>MAKKTGAKYPKSLLSLPLVGSLPFLPRHGHMHNNFFKLQKKYGPIYSVRMGTKTTVIVGHHQLAKEVLIKKGKDFSGRPQMATLDILSNNRKGIAFADSGAHWQLHRRLAMATFALFKDGDQKLEKIICQEISTLCDMLATHNGQSIDISFPVFVAVTNVISLICFNTSYKNGDPELNVIQNYNEGIIDNLSKDSLVDLVPWLKIFPNKTLEKLKSHVKIRNDLLNKILENYKEKFRSDSITNMLDTLMQAKMNSDNGNAGPDQDSELLSDNHILTTIGDIFGAGVETTTSVVKWTLAFLLHNPQVKKKLYEEIDQNVGFSRTPTI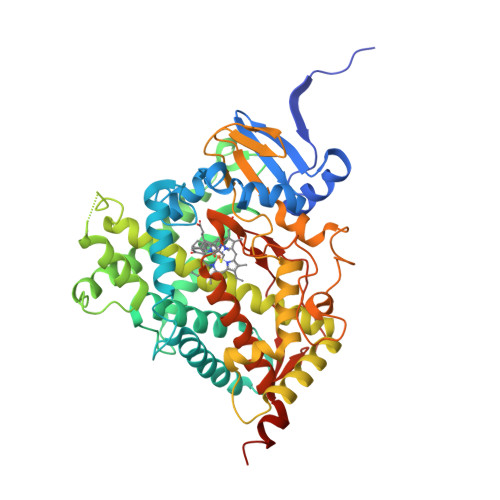SDRNRLLLLEATIREVLRLRPVAPMLIPHKANVDSSIGEFAVDKGTEVIINLWALHHNEKEWHQPDQFMPERFLNPAGTQLISPSVSYLPFGAGPRSCIGEILARQELFLIMAWLLQRFDLEVPDDGQLPSLEGIPKVVFLIDSFKVKIKVRQAWREAQAEGSTHHHH[4x]4-{[5-({(2S)-2-butyl-5-oxo-4-[3-(trifluoromethoxy)phenyl]piperazin-1-yl}methyl)-1H-imidazol-1-yl]methyl}benzonitrile 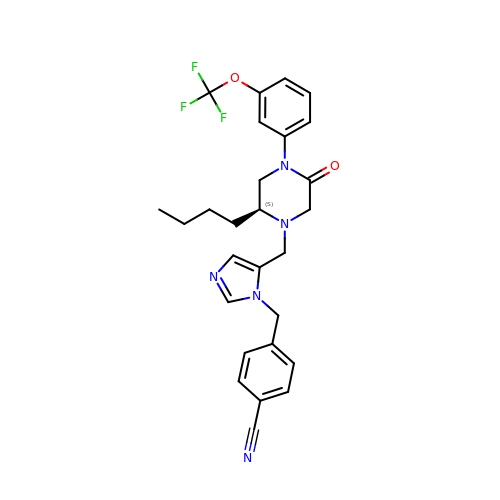| C27 H28 F3 N5 O2 | VSMQDFPGHHELTG-QHCPKHFHSA-N>[4x]SNAQEGTLERSDWRKFFSEFQAKGTIVVADERQADRAMLVFDPVRSKKRYS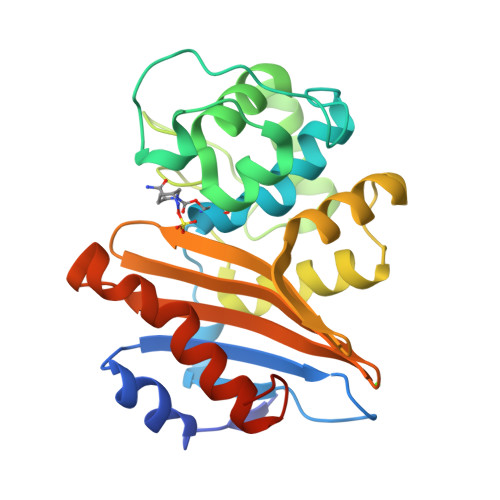PASTFKIPHTLFALDAGAVRDEFQIFRWDGVNRGFAGHNQDQDLRSAMRNSTVWVYELFAKEIGDDKARRYLKKIDYGNADPSTSNGDYWIEGSLAISAQEQIAFLRKLYRNELPFRVEHQRLVKDLMIVEAGRNWILRAKTGWEGRMGWWVGWVEWPTGSVFFALNIDTPNRMDDLFKREAIVRAILRSIEALPPNPAVNSDAAR> MLKRVEIFTDGSCLGNPGPGGYGAILRYRGREKTFSAGYERTTNNRMELMAAIVALEALKEHCEVILSTDSHYVRKGITEWIHNWKKRGWKKADKKPVKNVDLWKRLDAALGRHKIKWEWVKG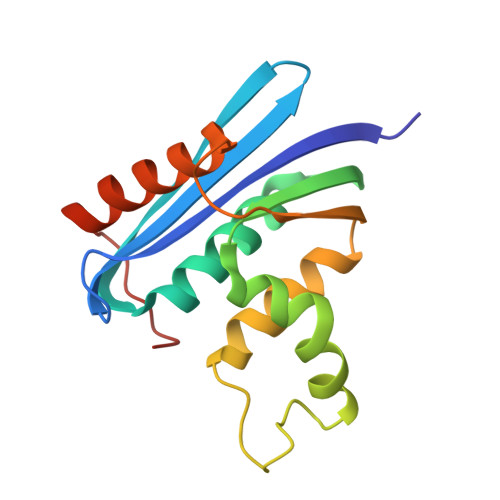HAGHPENERCDELARAAAMKPKLEDTGYQVEV>[2x]MASEDKNIIHGPPPFYSLDIGTAGEQLHKFMKKYAQITGTIAFTDAHNGVNVTYAEYFEMACRLAQSMKNYGLTLKHRIAVCSENSLQFFMPICGALFIGVGVAPTNDIYNERELYNSLGISQPTIVFCSKRALQKILGVQQKLPIIEKIIILDSQEDFMGKQSMNSFIRQFLPETFNEYDYVPDSFALNTTAFIMNSSGSTGLPKGVDLTHQNIVVRFSHCRDPIFGNQIIPDTSILSVIPFHHGFGMSTTLGYLVCGFRIVLMYRFEEELFLRSLQNYKCQSALLVPTLFSFFAKSTLVDKYDLSNLHEVASGGAPLAKEVGEAVAKRFNLVGIRQGYGLTETTSACIITPEGDNKPGACGKVVPFFSAKVTDLDTGKTLGPNQRGELWLKGPMVMKGYVNNPEATHSLIDKEGWVRTGDIAYYDEDEHFFIVDRLKSLIKYKGYQVPPAELESILLQHPYIFDAGVAGIPDPDAGELPAAVVVLEEGKTMTEKEVMDYVAGQVTSSKRLRGGVKFVDEVPKGLTGKIDGRKIREILLKAKKSKL

At the core of this natural phenomenon lies a fundamental process of energy transduction by luciferase enzymes that convert the chemical energy stored within the ground-state substrate (luciferin) to an excited, emissive state of the product (oxyluciferin) by a spin-forbidden process. Although beetle luciferase systems share identical substrates and chemical reaction sequence, they emit a range of different colors from yellow green (λmax ≈ 560 nm), which is typical for common firefly species, such as the North American firefly Photinus pyralis (GPp) and the Japanese firefly Luciola cruciata (GLc), to orange and even red (λmax = 590–623 nm) from certain click beetles and railroad worms. Here, we describe the first crystal structures of two rare WT luciferases from Brazilian beetles that emit light with exceptional colors; a luciferase from the head lanterns of the glow-worm P. hirtus (Coleoptera: Phengodidae), the only known luciferase that naturally emits red light (λmax = 623 nm; REPh), and a green-emitting luciferase from the firefly A. vivianii (Coleoptera: Lampyridae) that displays a blue-shifted emission relative to common firefly luciferases (λmax = 538 nm at pH 8; GBAv). Biochemical and structural analyses of the two luciferases, combined with computational modeling, provide the best insight yet into the relationship between the structure and color of light emitted by beetle luciferases.

To identify structural features that are important in the color tuning mechanism, the crystal structure of GBAv luciferase with a blue-shifted green emission of lmax = 538 nm at pH 8 was determined for comparison with the REPh. The GBAv crystals diffract to a resolution of 1.9 Å when free of substrate and crystallize in a space group P212121 with two independent GBAv monomers in the asymmetric unit. Although the N-terminal domains of the two GBAv molecules are very similar (root-mean-square deviation [RMSD] value of 0.1 Å calculated on all backbone atoms), their C-terminal domains have different conformations with an RMSD value of 2.1 Å. Thus, although the luciferase in both molecules can be considered as being in its “open” conformation, the luciferase with the smaller aperture is maybe an intermediate between the “open” and “closed” conformations, the latter being attributed to the structure of GLc in complex with the reaction products. We were able to discern with sufficient accuracy the structure of loop in both independent molecules in the crystal of GBAv, in which the open conformation is stabilized by interactions between T527 and K529 of loop, and D422 and D436 of the N-terminal domain. The structural integrity of loop is maintained by interaction between K524 and the backbone of G528. In GBAv, loop is tightly held by strong ionic interactions between E354 on the loop and R337 on the N-terminal domain. The ionic interactions on both sides of loop fix its position relative to the enzyme backbone.> MTNKLFEHTVLYDSGDAFFELKGNASMKLSPKAAIEVCNEAAKKGLWILGIDGGHWLNPGFRIDSSASWTYDMPEEYKSKIPENNRLAIENIKDDIENGYTAFIITLKM;> MLAKNKGKIPGLKIDQKIRGQMPERGWTEDDIKNTVSNGATGTSFDKRSPKKTPPDYLGR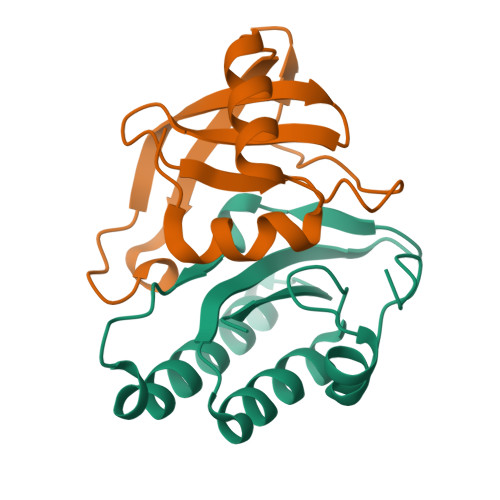NDPATVYGSPGKYVVVNDRTGEVTQISDKTDPGWVDDSRIQWGNKNDQ> MSTTLAIVRLDPGLPLPSRAHDGDAGVDLYSAEDVELAPGRRALVRTGVAVAVP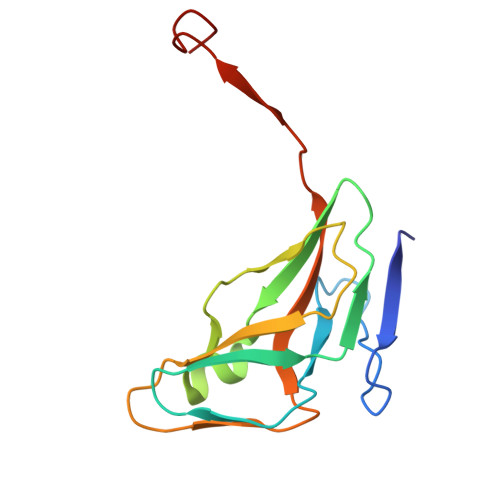FGMVGLVHPRSGLATRVGLSIVNSPGTIDAGYRGEIKVALINLDPAAPIVVHRGDRIAQLLVQRVELVELVEVSSFDEAGLA>[6x]GPMQTARDEIIQDPALAAGKYYAYEAPVSDKVSKAPAGYEPF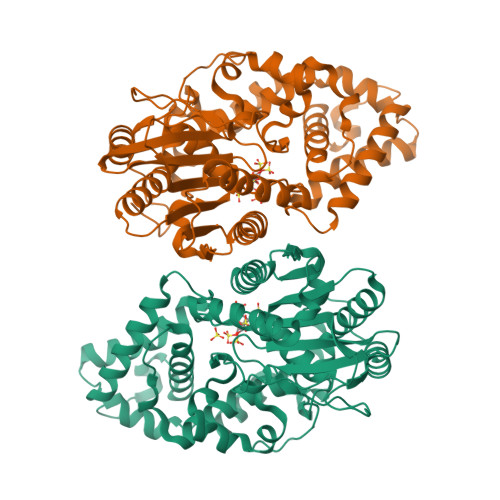YISAFARHGSRYLTDEEKYAEPVSVLRKADREGYLTTDGKKALQVMERLWKEAENRYGELTAKGAAQHQGLVERMYKHYPQVFVKGAHVDARSTYKTRAFLSMAAACVRLAQLNSGLLITQDASAHDAYYIKYKNKTFEQQHLAQSDSVYRIADSVYVHPARLMKQLFTRNVSAEELGVSPVVLMGELFELDGISQSSYGQEGLSFLFTDDERYDMWQRNNFEWYYEKGASPLSDCCMYHLERNLLENFIMTADTAIASPYRCVTLRYGHDTNLAPLAALMGMNRLQTETTDWQQIADTYRTYRIIPMCGNIQLIFYRRKGSSDILVKPLLNEREVTLPVETDCAPFYHWADVRAYWQKVADSIVLPDSGMQHD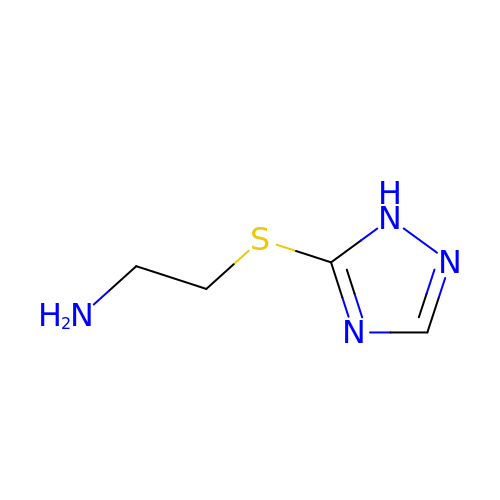2-(1H-1,2,4-triazol-5-ylsulfanyl)ethanamine | C4 H8 N4 S | VKHQZYSNDYRJDZ-UHFFFAOYSA-N>[2x]DEQPHIGNYRLLKTIGKGNFAKVKLARHILTGREVAIKIIDKTQLNPTSLQKLFREVRIMKI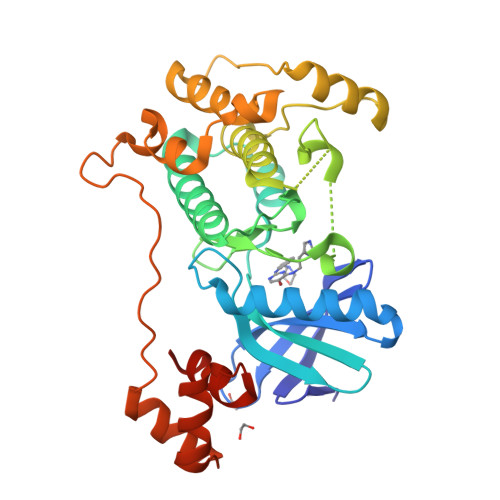LNHPNIVKLFEVIETEKTLYLIMEYASGGEVFDYLVAHGRMKEKEARSKFRQIVSAVQYCHQKRIVHRDLKAENLLLDADMNIKIADFGFSNEFTVGGKLDTFCGSPPYAAPELFQGKKYDGPEVDVWSLGVILYTLVSGSLPFDGQNLKELRERVLRGKYRIPFYMSTDCENLLKRFLVLNPIKRGTLEQIMKDRWINAGHEEDELKPFVEPELDISDQKRIDIMVGMGYSQEEIQESLSKMKYDEITATYLLLGRAENLYFQ>[4x]AAERIVVAGGSLTELIYAMGAGERVVGVDETTSYPPETAKLPHIGYWKQ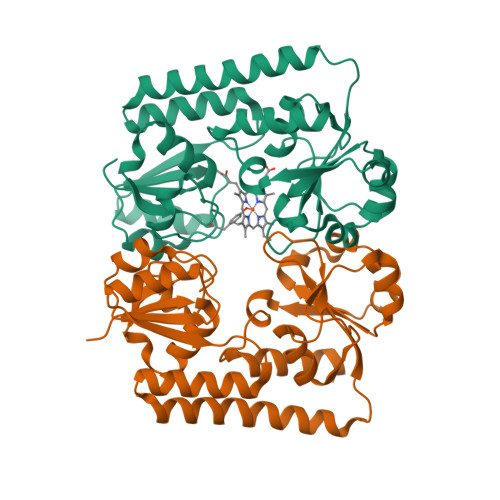LSSEGILSLRPDSVITWQDAGPQIVLDQLRAQKVNVVTLPRVPATLEQMYANIRQLAKTLQVPEQGDALVTQINQRLERVQQNVAAKKAPVKAMFILSAGGSAPQVAGKGSVADAILSLAGAENVATHQQYKSYSAESLIAANPEVIVVTSQMVDGDINRLRSIAGITHTAAWKNQRIITVDQNLILGMGPRIADVVESLHQQLWPQ>[2x]MILDTDYITENGKPVIRVFKKENGEFKIEYDRTFEPYFYALLKDDSAIEDVKKVTAKRHGTVVKVKRAEKVQKKFLGRPIEVWKLYFNHPQDVPAIRDRIRAHPAVVDIYEYDIPFAKRYLIDKGLIPMEGDEELTMLAF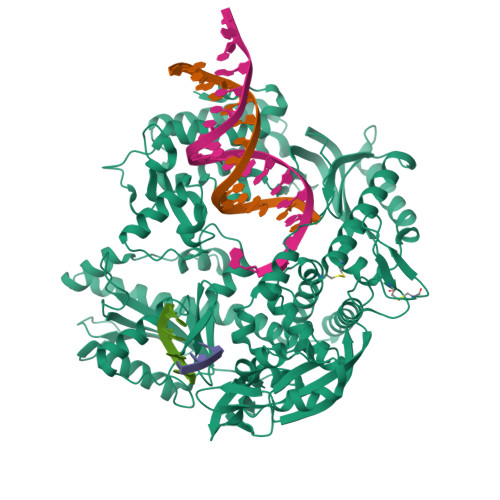AIATLYHEGEEFGTGPILMISYADGSEARVITWKKIDLPYVDVVSTEKEMIKRFLRVVREKDPDVLITYNGDNFDFAYLKKRCEELGIKFTLGRDGSEPKIQRMGDRFAVEVKGRIHFDLYPVIRRTINLPTYTLEAVYEAVFGKPKEKVYAEEIAQAWESGEGLERVARYSMEDAKVTYELGREFFPMEAQLSRLIGQSLWDVSRSSTGNLVEWFLLRKAYKRNELAPNKPDERELARRRGGYAGGYVKEPERGLWDNIVYLDFRSLYPSIIITHNVSPDTLNREGCKEYDVAPEVGHKFCKDFPGFIPSLLGDLLEERQKIKRKMKATVDPLEKKLLDYRQRLIKILANSFYGYYGYAKARWYCKECAESVTAWGREYIEMVIRELEEKFGFKVLYADTDGLHATIPGADAETVKKKAKEFLKYINPKLPGLLELEYEGFYVRGFFVTKKKYAVIDEEGKITTRGLEIVRRDWSEIAKETQARVLEAILKHGDVEEAVRIVKEVTEKLSKYEVPPEKLVIHEQITRDLRDYKATGPHVAVAKRLAARGVKIRPGTVISYIVLKGSGRIGDRAIPADEFDPTKHRYDAEYYIENQVLPAVERILKAFGYRKEDLRYQKTKQVGLGAWLKVKGKKLEHHHHHH> GTTGGATDA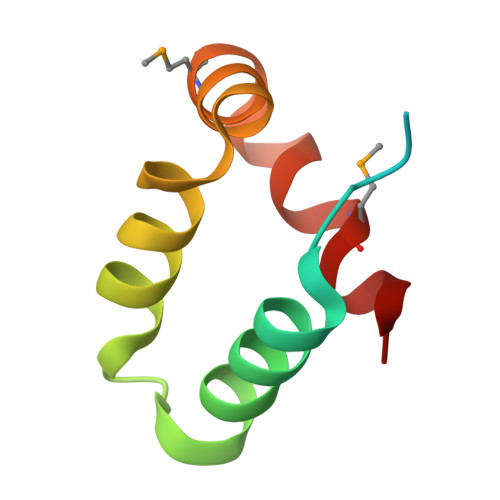AQGGPPGSIGLTVEDLLSLRQVVSGNPEALAPLLENISARYPQLREHIMANPEVFVSMLLEAV> KERQKVVEQMEHEMKEAAKALDFERAAELR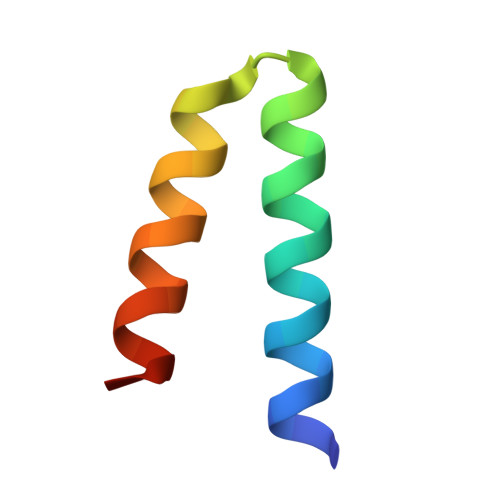DLLLELKAEG>[2x]TGHPYYLRSFLVVLKTVLE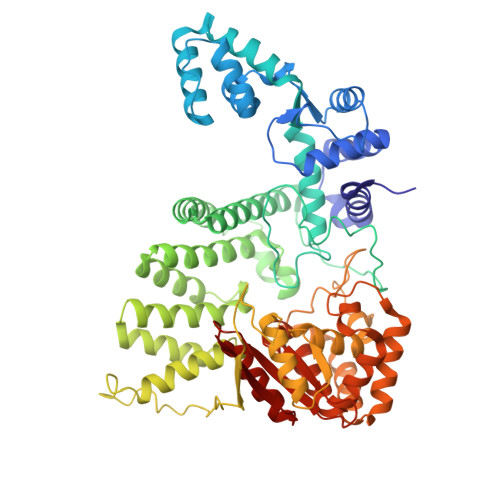NEDDMLLFDEQEKGIVTKFYQLSATGQKLYVRLFQRKLSWIKMTKLEYEEIALDLTPVIEELTNAGFLQTESELQELSEVLELLSAPELKSLAKTFHLVNPNGQKQQLVDAFLKLAKQRSVCTWGKNKPGIGAVILKRAKALAGQSVRICKGPRAVFSRILLLFSLTDSMEDEDAACGGQGQLSTVLLVNLGRMEFPSYTINRKTHIFQDRDDLIRYAAATHMLSDISSAMANGNWEEAKELAQCAKRDWNRLKNHPSLRCHEDLPLFLRCFTVGWIYTRILSRFVEILQRLHMYEEAVRELESLLSQRIYCPDSRGRWWDRLALNLHQHLKRLEPTIKCITEGLADPEVRTGHRLSLYQRAVRLRESPSCKKFKHLFQQLPEMAVQDVKHVTITGRLCPQRGMCKSVFVMEAGEAADPTTVLCSVEELALAHYRRSGFDQGIHGEGSTFSTLYGLLLWDIIFMDGIPDVFRNACQAFPLDLCTDSFFTSRRPALEARLQLIHDAPEESLRAWVAATWHEQEGRVASLVSWDRFTSLQQAQDLVSCLGGPVLSGVCRHLAADFRHCRGGLPDLVVWNSQSRHFKLVEVKGPNDRLSHKQMIWLAELQKLGAEVEVCHVVAV> 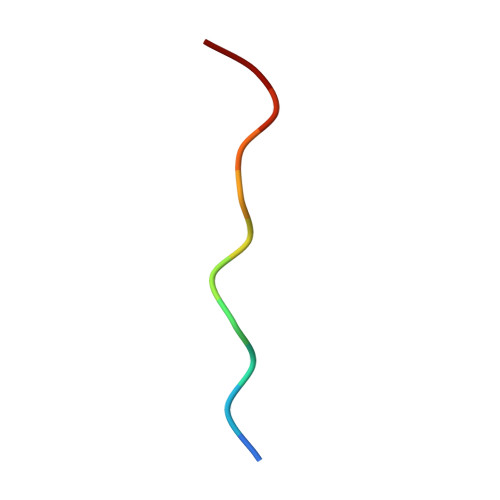LVKSKATNLLY~{N}-(3,5-dimethoxyphenyl)-4-methyl-3-[(1-methyl-6-pyridin-3-yl-pyrazolo[3,4-d]pyrimidin-4-yl)amino]benzamide | C27 H25 N7 O3 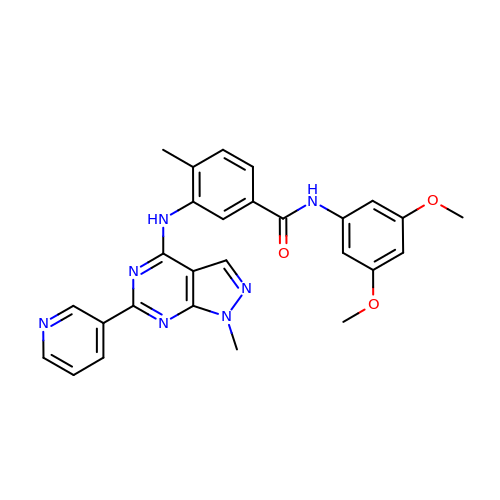| QUSRKKAMVTXFME-UHFFFAOYSA-N>GSHMSISEGDDAYIRSLIHFFGNQPDPWGIKDTKSVFIYANQPFRELVGMKNRNVEGLTDADMDCETAAFADSFQAQDRLVEQGREKKIVLDVHPYANGWRVFTFTKTPLIMPSGRVAGTIFHGQDLTDTAGRIERAVVELLLPSSGQAGSFETNVVGLNLTEREELVLFFL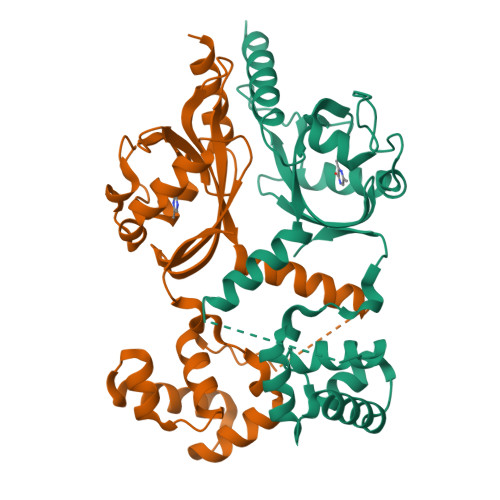LRGRTAKDIAGMLGRSPRTIEHAIERIRNKFGAGNKRELIDMAMSKGYYSMVPKALFHTQVSMLLK[2x]> GSDEKRLHFGNGHLKLPGLRTYVDPHTFEDPTQTVHEFAKELDATNISIDKVVGAGEFGEVCSGRLKLPSKKEISVAIKTLKVGYTEKQRRDFLGEASIMGQFDHPNIIRLEGVVTKSKPVMIVTEYMENGSLDSFLRKHDAQFTVIQLVGMLRGIASGMKYLSDMGYVHRDLAARNILINSNLVCKVSDFGLSRVLEDDPEAAYTTRGGKIPIRWTSPEAIAYRKFTS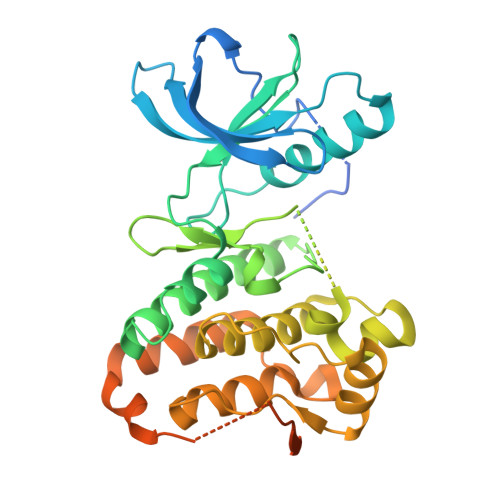ASDVWSYGIVLWEVMSYGERPYWEMSNQDVIKAVDEGYRLPPPMDCPAALYQLMLDCWQKDRNNRPKFEQIVSILDKLIRNPGSLKIITSAAARPSNLLLDQSNVDITTFRTTGDWLNGVWTAHCKEIFTGVEYSSCDTIAKIS>RGSHMETWVLGRRDVAEVVAAVGRDELMRRIIDRLTGGLAEIGRGERHLSPLRGGLERSEPVPGIWEWMPHREPGDHITLKTVGYSPANPARFGLPTILGTVARYDDTTGALTALMDGVLLTALRTGAASAVASRLLARPDSHTLGLIGTGAQAVTQLHALSLVLPLQRALVWDTDPAHRESFARRAAFTGVSVEIAEPARIAAEADVISTATSVAVGQGPVLPDTGVREHLHINAVGADLVGKTELPLGLLERAFVTADHPEQALREGECQQLSADRLGPQLAHLCADPAAAAG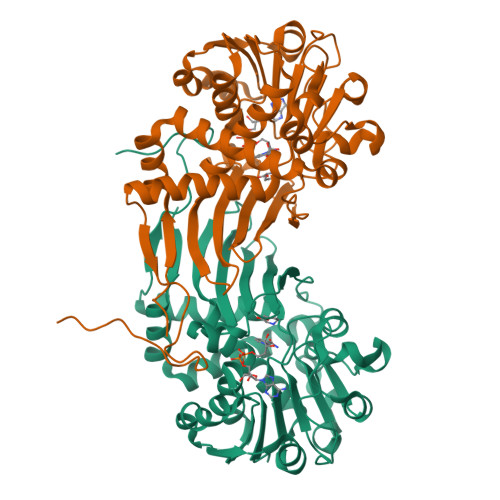RQDTLSVFDSTGFAFEDALAMEVFLEAAAERDLGIRVGIEHHPGDALDPYALQPLPLPLAAPAH[2x]>GPVDNWRDNLVRQVQHSELELVANFADIPLRLSQILKLKPGDVLPIEKPDRIIAHVDGVPVLTSQYGTVNGQYALRVEHLINPILNSLNEEQPKNNPSDENTGALDDLWADALNEQKATTTKSAADAVFQQLGGGDVSGAMQDIDLIMDIPVKLTVELGRTRMTIKELLRLTQGSVVALDGLAGEPLDILINGYLIAQGEVVVVADKYGVRITDIITPSERMRRLSR[2x];> VFQQLG;> GALDDLWADELGRT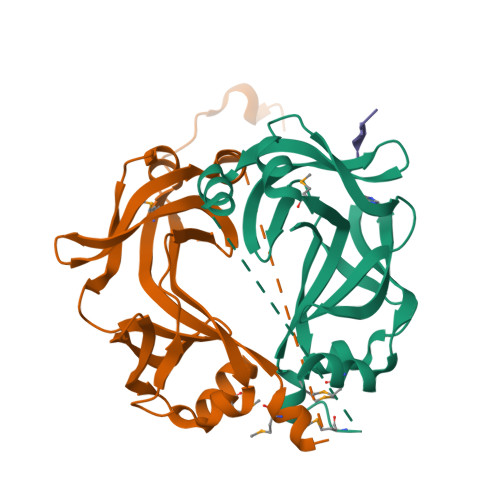RMTIKELLRLTQGSVVALDGLAGEPLDILINGYLIAQGEVVVVADKYGVRITDIITPSERMRRLSR> ARKREVRLMKNREAARESRRKKKEYVKCLENRVAVLENQNKTLIEELKALKDLYSHKSD;> SNPRKFSEKIALQKQRQAEETAAFEE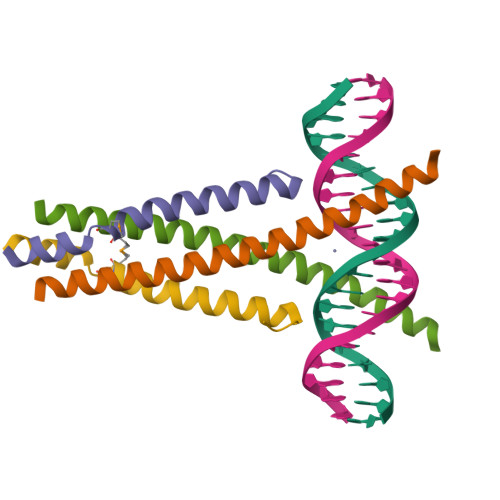VMMDIGSTRLQAQKLR>[2x]GAMDYTLRKIKIAAAHSLSLGLLPTIVKQMPTQFTYAVEAIDVDQA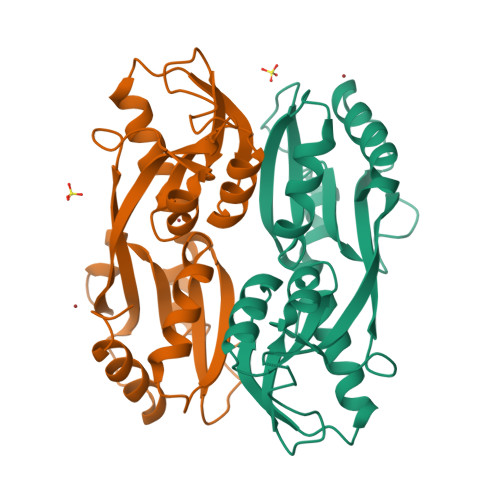VDMLREGQSDFIFSYHDENLQQAPFDNIRLFESRLFPVCANNGRGEPRYTLEQPHFPLLNYSQNSYMGRLINRTLTRHAELSFSTFFVSSMSELLKQVAMDGCGIAWLPEYAIRQEITDGRLIVLDADELVIPIQAYAYRMNTRMSQVAETFWRDLRGLQAAL>SNAMSEYRTVSAAAMLGTYEDFLELFEKGYEDKESVLKSNILYDVLRNNNDEARYKISMFLINKGADIKSRTKEGTTLFFPLFQGGGNDITGTTELCKIFLEKGADITALYKPYKIVVFKNIFNYFVDENEMIPLYKLIFSQSGLQLLIKDKWGLTALEFVKRCQKPIALKMMEDYIKKYNLKENS[2x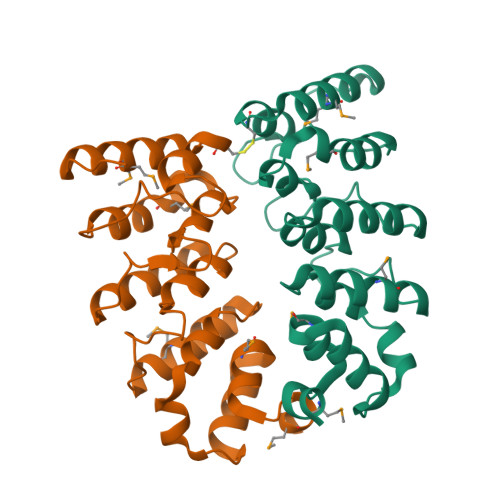]> GHMKHTIDPSSPDFQPIPSFEECFPKSTKEHKEVVHEESGHVLKVPFRRVHLSGGEPAFDNYDTSGPQNVNAHIGLAKLRKEWIDRREKLGTPRYTQMYYAKQGIITEEMLYCATREKLDPEFVRSEVARGRAIIPSNKKHLELEPMIVGRKFLVKVNANIGNSAVASSIEEEVYKVQWATMWGADTIMDLSTGRHIHETREWILRNSAVPVGTVPIYQALE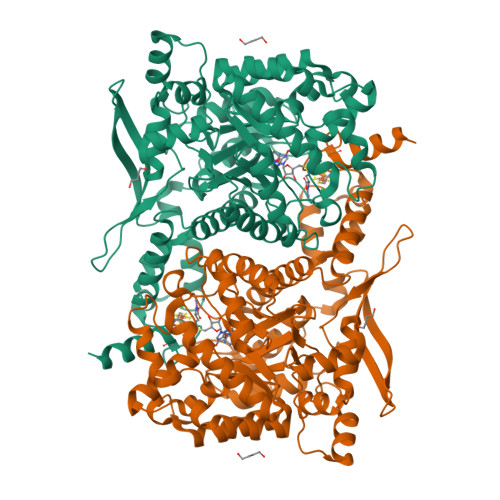KVDGIAENLNWEVFRETLIEQAEQGVDYFTIHAGVLLRYIPLTAKRLTGIVSRGGSIHAKWCLAYHKENFAYEHWDDILDICNQYDVALSIGDGLRPGSIYDANDTAQFAELLTQGELTRRAWEKDVQVMNEGPGHVPMHKIPENMQKQLEWCNEAPFYTLGPLTTDIAPGYDHITSAIGAANIGALGTALLCYVTPKEHLGLPNRDDVKAGVIAYKIAAHAADLAKQHPHAQAWDDALSKARFEFRWMDQFALSLDPMTAMSFHDETLPADGAKVAHFCSMCGPKFCSMKITEDIRKYAEENGYGSAEEAIRQGMDAMSEEFNIAKKTISGEQHGEVGGEIYLPESYVKAAQK>MHHHHHHMRGSMASEIHMTGPMC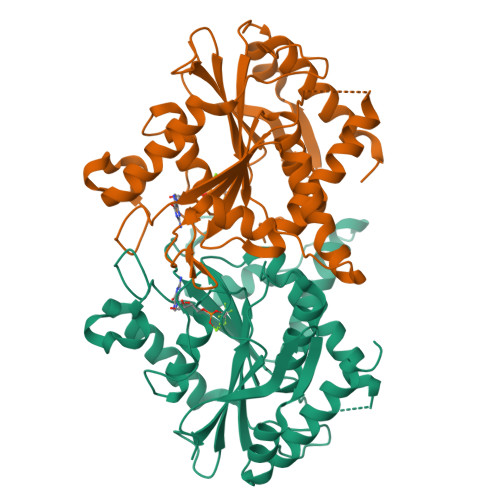LIENTNGRLMANPEALKILSAITQPMVVVAIVGLYRTGKSYLMNKLAGKKKGFSLGSTVQSHTKGIWMWCVPHPKKPGHILVLLDTEGLGDVEKGDNQNDSWIFALAVLLSSTFVYNSIGTINQQAMDQLYYVTELTHRIRSKSSPDENENEVEDSADFVSFFPDFVWTLRDFSLDLEADGQPLTPDEYLTYSLKLKKGTSQKDETFNLPRLCIRKFFPKKKCFVFDRPVHRRKLAQLEKLQDEELDPEFVQQVADFCSYIFSNSKTKTLSGGIQVNGPRLESLVLTYVNAISSGDLPCMENAVL[2x]4-oxidanylfuro[3,2-g]chromen-7-one | C11 H6 O4 | 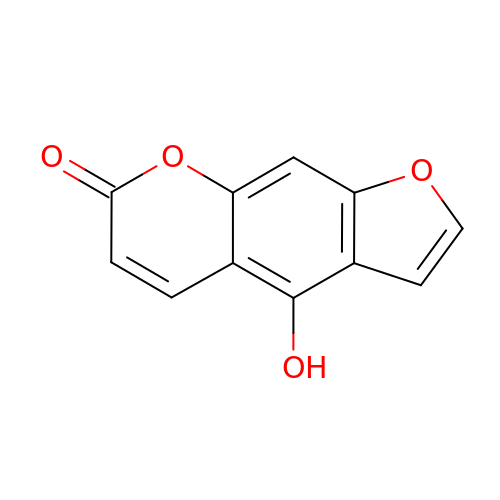GIJHDGJRTUSBJR-UHFFFAOYSA-N(4R,5S,6S)-3-{[(3S,5S)-5-(dimethylcarbamoyl)pyrrolidin-3-yl]sulfanyl}-6-[(1R)-1-hydroxyethyl]-4-methyl-7-oxo-1-azabicyclo[3.2.0]hept-2-ene-2-carboxylic 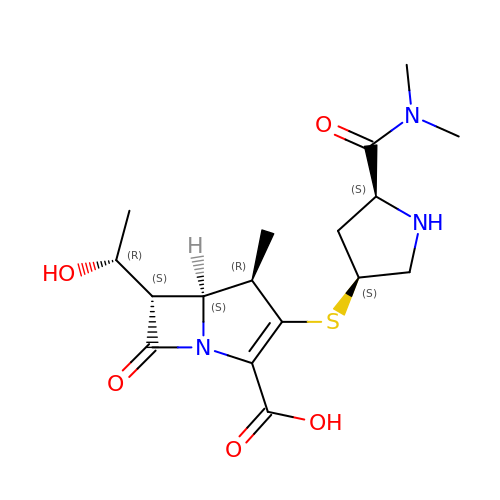acid | C17 H25 N3 O5 S | DMJNNHOOLUXYBV-PQTSNVLCSA-N Outer membrane porins (OMPs) are an important class of β-barrel proteins that form water-filled channels in Gram-negative bacteria. From a clinical perspective, OMPs are important in modulating the diffusion of antibiotics into the bacterial cell, where mutations or reduced expression of the OMPs enhance antibiotic resistance. It has also been shown that OMPs participate in F-like plasmid conjugation, a form of horizontal gene transfer where plasmids are transferred from donor to recipient bacteria in a contact-dependent manner. We have recently shown that the efficient conjugation of the multidrug-resistant R100-1 plasmid into both Escherichia coli (EC) and Klebsiella pneumoniae (KP) relies on the formation of mating-pair stabilization via interaction between the R100-1-encoded OM protein TraNα in the donor and the OMP OmpWEC or OmpWKP in the recipient. In addition to its role in conjugation, OmpW contributes to virulence as the upregulation of OmpWEC increases resistance to host immune defence.

Here, we present the crystal structure of OmpWKP at 3.2 Å resolution and draw structural comparisons with OmpWEC, both of which are conjugation receptors for TraNα. The structure of OmpWKP was solved by molecular replace­ment using the AlphaFold-predicted model. Continuous electron density could be observed for most of the structure except for Gly41–Phe52, which were omitted from model building. The OmpWKP structure consists of eight antiparallel β-strands (β1–β8) that arrange to form a hollow β-barrel in the OM and an extracellular solvent-exposed region. The extracellular region is formed from the extended β-strands of the barrel and a single α-helical turn (α1) connecting β5 and β6. A hydrophobic gate is present midway through the channel consisting of residues Leu89 and Trp188, as in OmpWEC, where the extracellular entrance to the channel is lined with hydrophobic residues. The extracellular loop 1 that connects β1 and β2 is missing in both the OmpWKP and the OmpWEC structures, suggesting a highly flexible structure. In the OmpWEC structure an LDAO molecule is bound at the extracellular region but loop 1 is not fully resolved, suggesting that the inherited flexibility cannot be stabilized upon its binding. This highly mobile structural element on the extracellular loop is likely to shield the hydrophobic face of the extracellular region and it could transiently open to recruit hydrophobic substrates.

> EAGEFFIRAGTATVRPTEGSDNVLGSLGSFNVSNNTQLGLTFTYMATDNIGVELLAATPFRHKVGTGPTGTIATVHQLPPTLMAQWYFGDAQSKVRPYVGAGINYTTFFNEDFNDTGKAAGLSDLSLKDSWGAAGQVGLDYLINRDWLLNMSVWYMDIDTDVKFKAGGVDQKVSTRLDPWVFMFSAGYRF>GSMQNRQVANATKVAVAGASGYAGGEILRLLLGHPAYADGRLRIGALTAATSAGSTLGEHHPHLTPLAHRVVEPTEAAVLGGHDAVFLALPHGHSAVLAQQLSPETLIIDCGADFRLTDAAVWERFYGSSHAGSWPYGLPELPGARDQLRGTRRIAVPGCYPTAALLALFPALAADLIEPAVTVVAVSGTSGAGRAATTDLLGAEVIGSARAYNIAGVHRHTPEIAQGLRAVTDRDVSVSFTPVLIPASRGILATCTARTRSP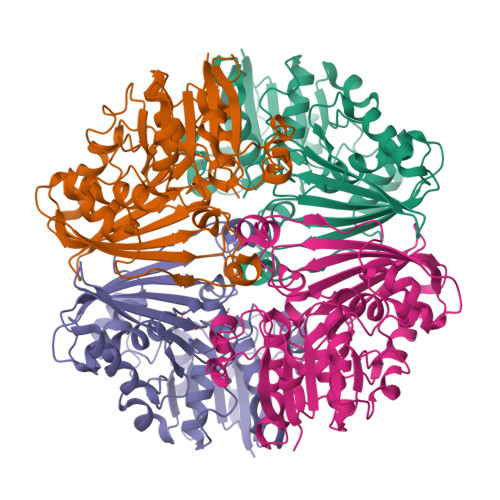LSQLRAAYEKAYHAEPFIYLMPEGQLPRTGAVIGSNAAHIAVAVDEDAQTFVAIAAIDNLVKGTAGAAVQSMNLALGWPETDGLSVVGVAP[8x]>MEYFNNINEYFNSINDSKILSLQNKKNTLMDTSGYNAEVRVEGNVQLNPIFPFDFKLGSSGDDRGKVIVTQNENIVYNAMYESFSISFWIRINKWVSNLPGYTIIDSVKNNSGWSIGIISNFLVFTLKQNENSEQDINFSYDISKNAAGYNKWFFVTITTNMMGNMMIYINGKLIDTIKVKELTGINFSKTITFQMNKIPNTGLITSDSDNINMWIRDFYIFAKELDDKDINILFNSLQYTNVVKDYWGNDLRYDKEYYMINVNYMNRYMSKKGNGIVFNTRKNNNDFNEGYKIIIKRIRGNTNDTRVRGENVLYFNTTIDNKQYSLGMYKPSRNLGTDLVP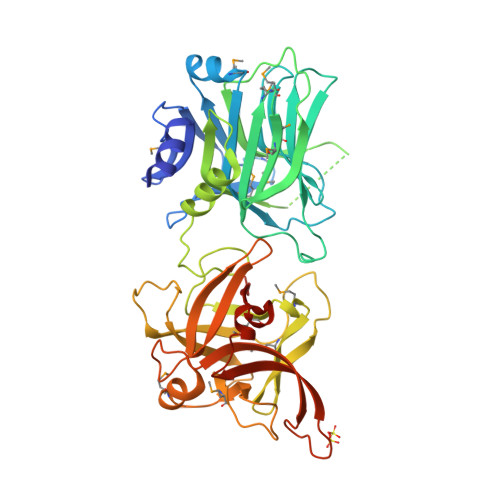LGALDQPMDEIRKYGSFIIQPCNTFDYYASQLFLSSNATTNRLGILSIGSYSFKLGDDYWFNHEYLIPVIKIEHYASLLESTSTHWVFVPASELEHHHHHH[2x]>[4x]MSNEIPKPVAPAPDILR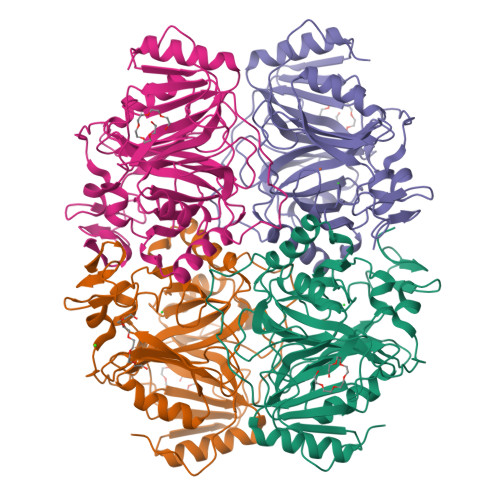CAYAELVVTDLAKSRNFYVDVLGLHVSYEDENQIYLRSFEEFIHHNLVLTKGPVAALKAMAFRVRTPEDVDKAEAYYQELGCRTERRKDGFVKGIGDALRVEDPLGFPYEFFFETTHVERLHMRYDLYSAGELVRLDHFNQVTPDVPRGRKYLEDLGFRVTEDIQDDEGTTYAAWMHRKGTVEDTALTGGNGPRLHHVAFSTHEKHNIIQICDKMGALRISDRIERGPGRHGVSNAFYLYILDPDNHRIEIYTQDYYTGDPDNPTITWNVHDNQRRDWWGNPVVPSWYTEASKVLDLDGNVQEIIERTDDSELEVTIGADGFSFTRAGDEDGSYHGQASKGFKLGNQL>[4x]SEFELRRQASMGLPKKALKESQLQFLTAGTAVSDSSHQTYKVSFIENGVIKNAFYKKLDPKNHYPELLAKISVAVSLFKRIFQGRRSAEERLVFDDEERLVGTLSISVDGFKGFNFHKESVPQESSAKEQVIPSTRTLIEKSFMEILLGRWFLDDDDGHPHNLSLAGDIDFDMFFYWFTIYMKEPRPAIGIPKTRVNLTVRDWEGFPNVKDSKPFHWPTYKNPGQETLPTVLPVQDKLVNLILEKTYPDPGQFEQLAHEPVAQEQKFAAALKILLTYQPEMIRKRLTELFGEMTLNYT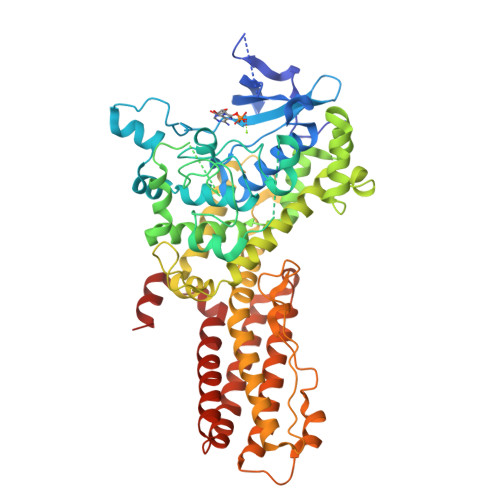SLDETDVALRNQYEKTFPHLCNENTNIKPFVDFIMNLYQMHYDNLYRVVVFYMGCENNGYGVPLPATNSALYHKPSFYKDIVEWARTQNITIFSKDDSSIKFDEDELRRRYHQVWRDAYAPTFRDLLHDSYSLTNKLLQQVSTFHVVLDEVEGKKPTDDTLTNAWELFGTMPELSLEKITPLISVDKDSKLRTALILLVEFTTQFHAVAKTYYQKDRKDLTEEDNLEFSEQLVQLYTNYNLKIRQSLAHTSTLAGEFNRIAVGLKQYTERANFQLHLTTTDEQMKEATVATT> TELTVDQQTLLDYIMDSYSKQRMPQEITNKILKEEFSAEENFLILTEMATSHVQILVEFTKRLPGFQTLDHEDQIALLKGSAVEAMFLRSAEIFNKKLPAGHADLLEERIRKSGISDEYITPMFSFYKSVGELKMTQEEYAL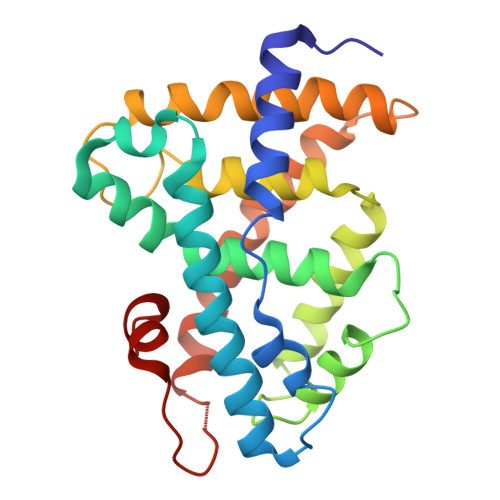LTAIVILSPDRQYIKDREAVEKLQEPLLDVLQKLCKIYQPENPQHFACLLGRLTELRTFNHHHAEMLMSWRVNDHKFTPLLCEIWDV> PTLWPQREALKSALQYPALAGPVFDALTVEGFTHPEYAAVRAAIDTAGGTSA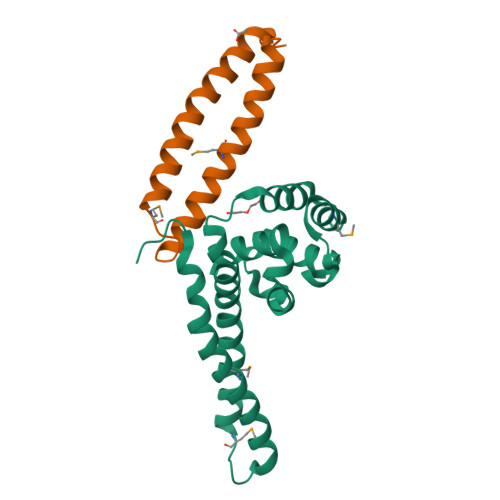GLSGAQWLDMVRQQTTSTVTSALISELGVEAIQVDDDKLPRYIAGVLARLQEVWLGRQIAEVKSKLQRMSPIEQGDEYHALFGDLVAMEAYRRSLLEQASGDDLHHHHHH;> DDKLPRYIAGVLARLQEVWLGRQIAEVKSKLQRMSPIEQGDEYHALFGDLVAMEAYRRSLLEQASGDDLHH>[2x]MLQKLIQILRRNEYVKNVYKNTVSNFIETSIPEITPFNARTS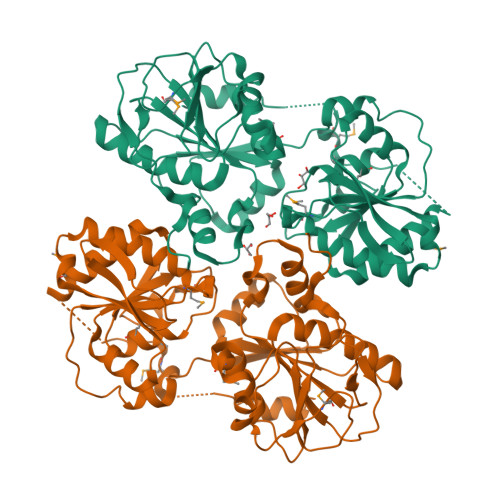SIKGKRLNLLVPSINQEHMFGGISTALKLFEQFDNKKFKKRIILTDATPNPKDLQSFKSFKYVMPEEDKDFALQIVPFNDRYNRTIPVAKHDIFIATAWWTAYAAQRIVSWQSDTYGIPPNKILYIIQDFEPGFYQWSSQYVLAESTYKYRGPQIAVFNSELLKQYFNNKGYNFTDEYFFQPKINTTLKNYINDKRQKEKIILVYGRPSVKRNAFTLIVEALKIFVQKYDRSNEWKIISVGEKHKDIALGKGIHLNSLGKLTLEDYADLLKRSSIGISLMISPHPSYPPLEMAHFGLRVITNKYENKDLSNWHSNIVSLEQLNPENIAETLVELCMSFNNRDVDKKESSNMMFYINEFNEFSFIKEIEEKL>SDPKLTKAVDSICDQFIVTKSKISQLTEYFIDCMEKGLEPCENKGLPMIPTFVTDKPSGQEHGVTMLAADLGGTNFRVCSVELLGNHEFKIEQEKSKIPTFFFQDDHHVTSKDLFQHMALITHQFLTKHHKDVIQDYKWKMGFTFSYPVDQTSLSSGKLIRWTKGFKIGDTVGQDVVQLFQQELNDIGLSNVHVVALTNDTTGTLLARCYASSDAARAINEPVIGCIFGTGTNGCYMEKLENIHKLDPASREELLSQGKTHMCINTEWGSFDNELNHLPTTSYDIKIDQQFSTNPGFHLFE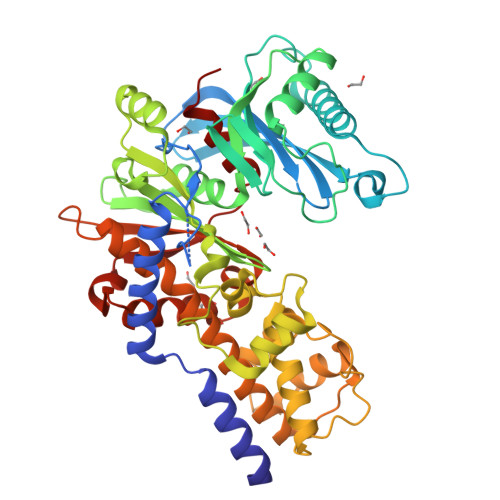KRVSGLYLGEILRNILLDLEKQELFDLKESVLKNNPFILTTETLSHIEIDTVENDLQDTRDALLKAADLETTFEERVLIQKLVRAISRRAAFLAAVPIAAILIKTNALNQSYHCQVEVGCDGSVVEHYPGFRSMMRHALALSPIGPEGERDVHLRISKDGSGVGAALCALHANY[3x]> DSSIKRTANINLYKLDQRFKQSRINIESFHSTVLLTGQVPDPYLKQLAEDNVKAMSDVKAVHNYITVGNKVSYNTIMQDAGVTANTRALLMKAPVVSDSKVLVHTEDGVLYVMGRLNTAEINDLNNVLQNVGNVTKIVTLIDNIDLAPAPAASTASATTTPVINNVLAQPTVQTPVAIDPDQTDPASSAQ

A recent study showed that A. baumannii upregulates production of an outer membrane lipoprotein, which we designate BonA, in response to challenge with polymyxins. Analyses through X-ray crystallography, small-angle X-ray scattering, electron microscopy, and multiangle light scattering demonstrate that BonA has a dual BON (Bacterial OsmY and Nodulation) domain architecture and forms a decamer via an unusual oligomerization mechanism. BonA from A. baumannii is a member of a diverse family of dual-BON domain outer membrane lipoproteins. We demonstrate that BonA is anchored to the outer membrane where it plays a role in maintaining membrane structure and is required for twitching motility.

High-quality crystals were only obtained for N-terminally truncated BonA, missing the 27 amino acids (aa) after its lipid-anchoring cystine. The structure of this protein, designated BonA-27N, was solved at 1.65 Å by single-wavelength anomalous dispersion (SAD) phasing, using selenomethionine labeled protein. The crystal structure of BonA-27N consists of two α/β-sandwich BON domains that interact extensively via the external face of their three-strand β-sheets. In contrast to the structure of DolP in which both domains adopt a canonical BON domain fold, in the BonA structure, α-helix 1 (αH1) of BON domain 1 (BON1) does not adopt the expected BON domain conformation of running parallel to the BON domain β-sheet. Rather, it is displaced from the rest of the domain. The 39 aa of the C-terminal extension of BonA-27N (aa 196 to 235) are disordered in the crystal structure. Analysis of BonA-27N crystallographic symmetry reveals that it exists as a dimer, aligned with the crystallographic 2-fold axis. The interface is stabilized by αH1 of BON domain 2 (BON2), which substitutes for the displaced αH1 of BON1, thus completing the α/β-sandwich fold of BON1. This interaction of αH1 of BON2 with BON1 is largely mediated by hydrophobic interactions, with Tyr118 and Met122 of αH1 of BON2 extending deeply into a hydrophobic pocket created by the displacement of αH1 of BON1. The interface also contains two symmetrical, highly solvated pockets, which trap a total of 34 water molecules, as well as two Zn2+ ions which were present at a high concentration in the crystallization solution.1-[(1S)-4-carbamimidamido-1-carboxybutyl]-5-oxo-D-proline | C11 H18 N4 O5 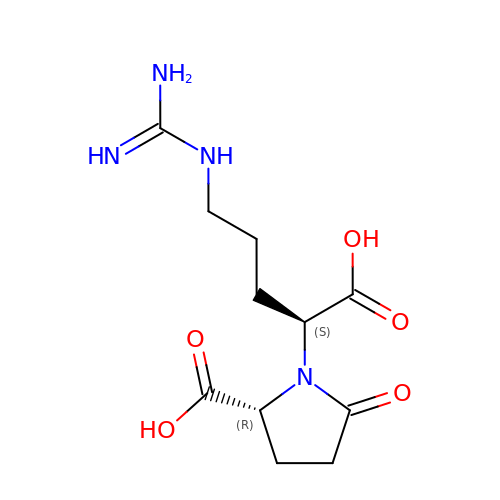| GTRMYGUJZGMZEF-NKWVEPMBSA-N N-(2-phenylethyl)methanesulfonamide 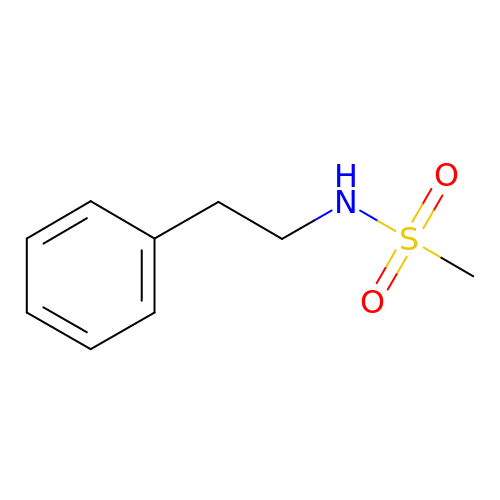| C9 H13 N O2 S | JGDDFCYMSLNOGJ-UHFFFAOYSA-N> GASGDLYEVERIVDKRKNKKGKWEYLIRWKGYGSTEDTWEPEHHLLHCEEFIDE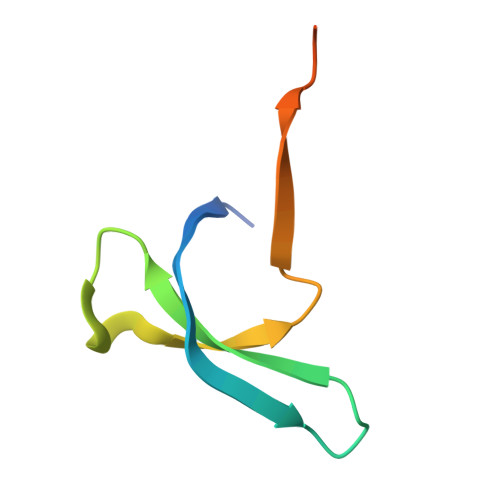FNGLHMSK TOLUENE | C7 H8 | 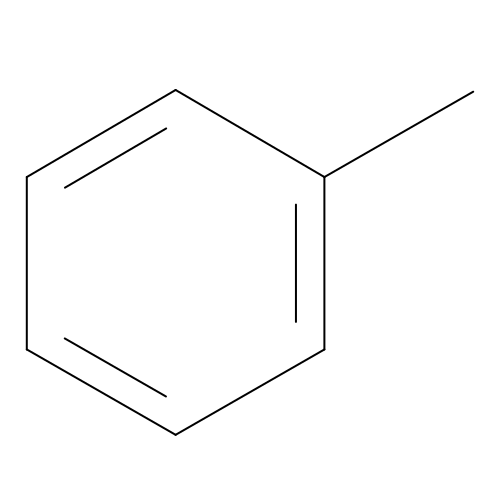YXFVVABEGXRONW-UHFFFAOYSA-N> PMQS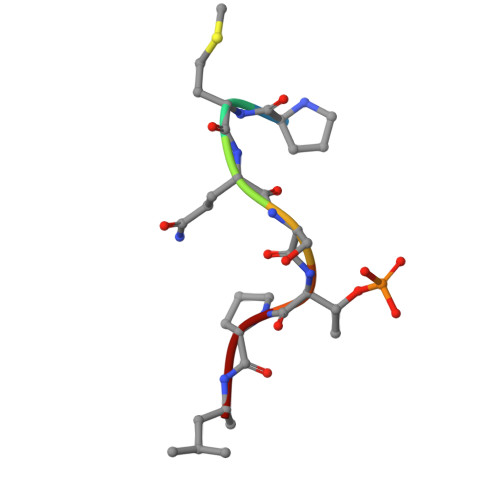TPL TMEM106B is a type II transmembrane protein of 274 residues that localizes to late endosomes and lysosomes. Here we used structure determination by cryogenic electron microscopy to show that residues 120–254 of the lysosomal type II transmembrane protein 106B (TMEM106B) also form amyloid filaments in human brains. The TMEM106B folds shared a similar five-layered ordered core comprising residues S120–G254 and contained 17 β-strands, each ranging between 3 and 15 residues. We observed three TMEM106B folds, with no clear relationships between folds and diseases.

We also determined the structures of filaments comprising two protofilaments of fold I, related by C2 symmetry. In all three folds, residues G177–N183 adopt a conserved conformation, with the positively charged residues K178 and R180 pointing outwards. In filaments made of two protofilaments with fold I, two pairs of these residues are on opposite sides of a contiguous extra density that runs along the helical symmetry axis. As the cofactor responsible for this density probably does not obey the imposed helical symmetry, the map in this region is of insufficient quality to allow its identification. In fold I, this region packs loosely against the other side of the C-terminal hairpin-like region with the formation of three large amphipathic cavities. Individuals with fold I were homozygous for T185 or S185, or heterozygous, indicating that fold I can accommodate a threonine or a serine at position 185. Filaments with fold I were more common than filaments with folds II or III.

>MGKSLSHLPLHSSKEDAYDGVTSENMRNGLVNSEVHNEDGRNGDVSQFPYVEFTGRDSVTCPTCQGTGRIPRGQENQLVALIPYSDQRLRPRRTKLYVMASVFVCLLLSGLAVFFLFPRSIDVKYIGVKSAYVSYDVQKRTIYLNITNTLNITNNNYYSVEVENITAQVQFSKTVIGKARLNNITIIGPLDMKQIDYTVPTVIAEEMSYMYDFCTLISIKVHNIVLMMQVTVTTTYFGHSEQISQERYQYVDCGRNTTYQLGQSEYLNVLQPQQ[6x]>DYKDDDDKLDRADILYNIRQTSRPDVIPTQRDRPVAVSVSLKFINILEVNEITNEVDVVFWQQTTWSDRTLAWNSSHSPDQVSVPISSLWVPDLAAYNAISKPEVLTPQLARVVSDGEVLYMPSIRQRFSCDVSGVDTESGA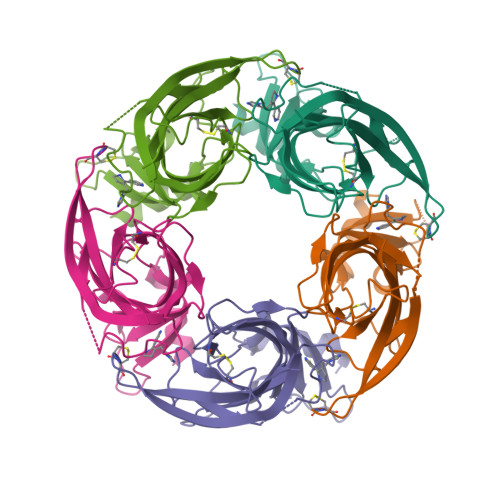TCRIKIGSWTHHSREISVDPTTENSDDSEYFSQYSRFEILDVTQKKNSVTYSCCPEAYEDVEVSLNFRKKGRSEIL[5x]N-(4-fluorophenyl)-4,5-dihydro-1H-imidazol-2-amine 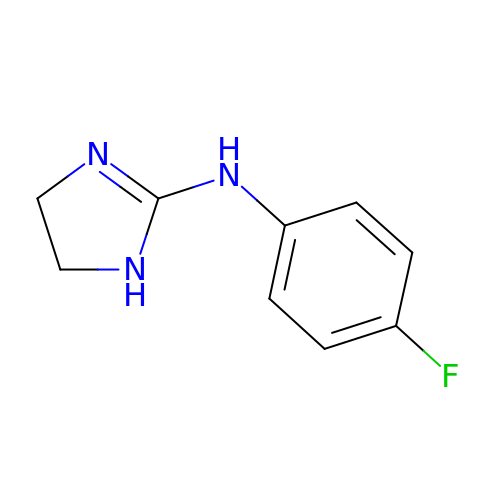| C9 H10 F N3 | IOUVWAKVDFTALH-UHFFFAOYSA-N NoV VP1 can be divided into two major domains: the N-terminal shell (S) domain and the C-terminal protruding (P) domain. The P domains form the outermost, dimeric protrusions of NoV virions, which plays critical roles in receptor recognition and host immune responses. HuNoVs recognize human histo-blood group antigens (HBGAs) as host receptors or attachment factors that play an important role in huNoV host susceptibility. In this study, we provided both phenotypic and structural evidence to show that huNoV DSV and VA115 recognize a group of glycans with terminal galactoses as ligands.

The results showed that two oligosaccharides (117 and 373) bound well to both DSV/VA115 P-GST fusion proteins with significantly higher binding signals compared with the remaining 583 oligosaccharides. Interestingly, only one oligosaccharide molecule bound in each asymmetric unit of the complex structures, since the remaining oligosaccharide binding pockets contain steric hindrance for oligosaccharides at crystal packing interface. The positions of the glycan binding pockets were located at the outermost surface of the P protein near the interface between the two P monomers, similar to the typical HBGA binding sites of other GI huNoVs. In DSV P protein, four amino acids D332, H334, S388 and P389 form the “bottom” of the binding interface, while residues Q393 and H396 constitute a side “wall,” S346′ and T344′ from the other monomer form the opposite “wall” (Fig. 3A– D). In DSV the Gal interacts with all four conserved amino acids (D332, H334, S388, and P389), as well as a variable residue Q393, forming eight or seven direct hydrogen bonds. Additionally, the Gal indirectly interacts with H396 and S346′ through water molecules. Similarly, mutations D332A and S388A of DSV resulted in loss of the glycan binding ability, while mutations H334A and Q393A of DSV reduced the binding affinity. Mutation P389A of DSV also retains nearly full glycan binding ability, since this residue interacts with the trisaccharide through the main chain carbonyl group. The structural data showed that the two GI.3 huNoVs bound non-HBGA glycans using terminal Gal as the MaBS, explaining the mechanism why these huNoVs could not bind HBGAs.

>GPLGSPEFQKTKPFSVPNLPLNTLSNSRVPSLINAMMISRDHGQMVQFQNGRVTLDGQLQGTTPTSLSQLCKIRGKVFHASGGNGLNLTELDGSAYHAFESPAPIGFPDIGDCDWHMSATATNNFTGSSNEYQILIKQESAFAPHLGHVQADNLSAGANTDLIVSLSWISPVSDQHRHDVDPWVIPRYGSSLTEAAQLAPPIYPPGFGEAIVFFMSDFPVVSGVNGMRIPCTLPQEYVAHFVNEQAPTRGEAALLHYVDPDTHRNLGEFKMYPEGFMTCVPNSSGSGPQTLPINGVFTFVSWVSRFYQLKPVGTAGPARRLGIRRS[2x]>[4x]MNMYSMPGYFQNMPTIGKELVNPNPENEQEIKAVESDIHESIKKALDAGITSEEKLNERGQLSAMQRINALIDPGTWCPLNSLFNPENNKFGTTNIVNGLGRVDGKWVYIVASDNKKMAGAWVPGQAENLIRCSDAAKMMHLPLIYLLNCSGVEFPNQDKVYPNRRGGGTPFFRNSELNQLGIPVIVGIYGTNPAGGGYHSISPTILIAHQDANMAVGGAGILSGMN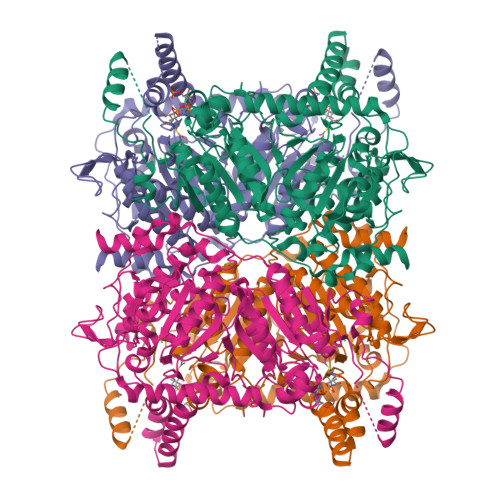PKGYIDDEAAEQIIAAQIENSKLKVPAPGSVPIHYDETGFFREVYQNDLGVIDGIKKYISYLPAYNLEFFRVDTPKAPQLPAEDLYSIIPMNQKRPYDIYEVIARLFDNSEFSEYKKGYGPEMVTGLAKVNGLLVGVIANVQGLLMNYPEYKQNSVGIGGKLYRQGLIKMNEFVTLCARDRIPLIWLQDTTGIDVGDEAEKAELLGLGQSLIYSIENSKLPSLEITIRKASAAAHYVLGGPQGNNTNVFSIGTGACEYYVMPGETAANAMYSRKLVKAKKAGEDLQPIIGKMNDMIQMYTDKSRPKYCTEKGMVDEIVDMTEVRPYIQAFTEAAYQNPQSICPMHQMLTPRSTREFETFGK5-CHLORO-THIOPHENE-2-CARBOXYLIC ACID ((3S,4S)-4-FLUORO- 1-{[2-FLUORO-4-(2-OXO-2H-PYRIDIN-1-YL)-PHENYLCARBAMOYL]-METHYL}-PYRROLIDIN-3-YL)-AMIDE 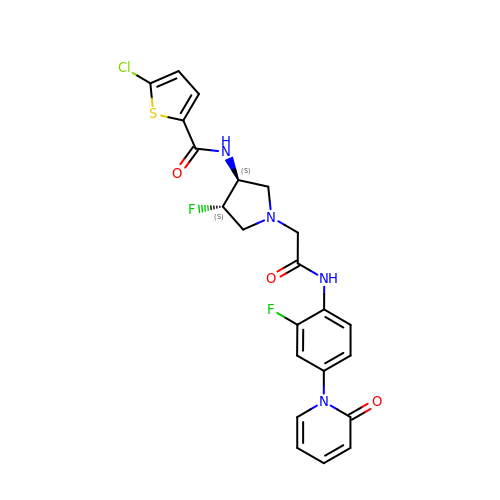| C22 H19 Cl F2 N4 O3 S | SXIYSYYSKHUTQQ-RDJZCZTQSA-N>[4x]RCPLMVKILDAVKGTPAGSVALKVSQKTADGGWT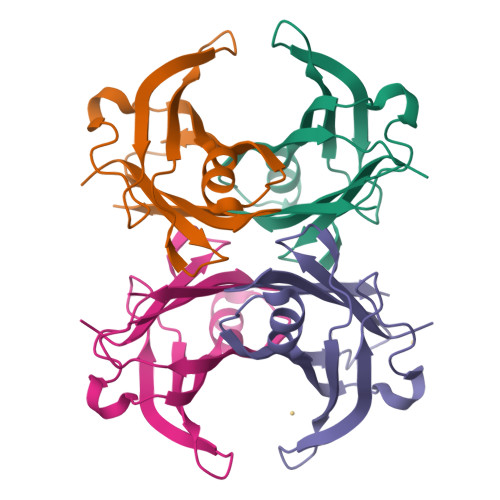QIATGVTDATGEIHNLITEQQFPAGVYRVEFDTKAYWTNQGSTPFHEVAEVVFDAHPEGHGHYTLALLLSPFSYTTTAVVSSVHE> CFCDHYAWTQWTSCSKTCNSGTQSRHRQIVVDKYYQENFCEQICSKQETRECNWQRCPINCLLGDFGPWSDCDPCIEKQSKVRSVLRPSQFGGQPCTAPLVAFQPCIPSKLCKIEEADCKNKFRCDSGRCIARKLECNGENDCGDNSDERDCGRTKAVCTRKYNPIPSVQLMGNGFHFLAGEPRGEVLDNSFTGGICKTVKSSRTSNPYRVPANLENVGFEVQTAEDDLKTDFYKDLTSLGHNENQQGSFSSQGGSSFSVPIFYSSKRSENINHNSAFKQAIQASHKKDSSFIRIHKVMKVLNFTTKAKDLHLSDVFLKALNHLPLEYNSALYSRIFDDFGTHYFTSGSLGGVYDLLYQFSSEELKNSGLTEEEAKHCVRIETKKRVLFAKKTKVEHRCTTNKLSEKHEGSFIQG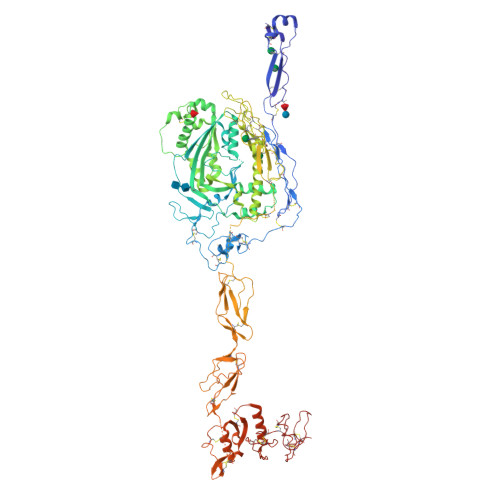AEKSISLIRGGRSEYGAALAWEKGSSGLEEKTFSEWLESVKENPAVIDFELAPIVDLVRNIPCAVTKRNNLRKALQEYAAKFDPCQCAPCPNNGRPTLSGTECLCVCQSGTYGENCEKQSPDYKSNAVDGQWGCWSSWSTCDATYKRSRTRECNNPAPQRGGKRCEGEKRQEEDCTFSIMENNGQPCINDDEEMKEVDLPEIEADSGCPQPVPPENGFIRNEKQLYLVGEDVEISCLTGFETVGYQYFRCLPDGTWRQGDVECQRTECIKPVVQEVLTITPFQRLYRIGESIELTCPKGFVVAGPSRYTCQGNSWTPPISNSLTCEKDTLTKLKGHCQLGQKQSGSECICMSPEEDCSHHSEDLCVFDTDSNDYFTSPACKFLAEKCLNNQQLHFLHIGSCQDGRQLEWGLERTRLSSNSTKKESCGYDTCYDWEKCSASTSKCVCLLPPQCFKGGNQLYCVKMGSSTSEKTLNICEVGTIRCANRKMEILHPGKCLA>MFCEKAMELIRELHRAPEGQLPAFNEDGLRQVLEEMKALYEQNQSDVNEAKSGGRSDLIPTIKFRHCSLLRNRRCTVAYLYDRLLRIRALRWEYGSVLPNALRFHMAAEEMEWFNNYKRSLATYMRSLGGDEGLDITQDMKPPKSLYIE[2x];>[2x]MDAAEVEFLAEKELVTIIPNFSLDKIYLIGGDLGPFNPGLPVEVPLWLAINLKQRQKCRLLPPEWMDVEKLEKMRDHERKEETFTPMPSPYYMELTKLLLNHASDNIPKADEIRTLVKDMWDTRIAKLRVSADSFVRQQEAHAKLDNLTLMEINTSGTFLTQALNHMYKLRTNLQPLESTQSQDF;>GPHMSEAYFRVESGALGPEENFLSLDDILMSHEKLPVRTETAMPRLGAFFLER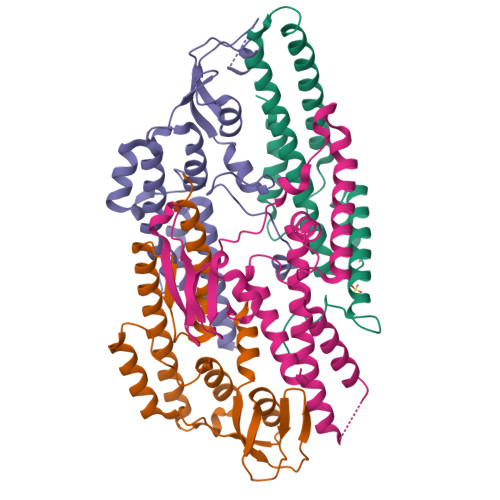SAGAETDNAVPQGSKLELPLWLAKGLFDNKRRILSVELPKIYQEGWRTVFSADPNVVDLHKMGPHFYGFGSQLLHFDSPENADISQSLLQTFIGRFRRIMDSSQNAYNEDTSALVARLDEMERGLFQTGQKGLNDFQCWEKGQASQITASNLVQNYKKRKFTDMED[2x];>MTEEVDFLGQDSDGGSEEVVLTPAELIERLEQAWMNEKFAPELLESKPEIVECVMEQLEHMEENLRRAKREDLKVSIHQMEMERIRYVLSSYLRCRLMKIEKFFPHVLEKEKTRPEGEPSSLSPEELAFAREFMANTESYLKNVALKHMPPNLQKVDLFRAVPKPDLDSYVFLRVRERQENILVEPDTDEQRDYVIDLEKGSQHLIRYKTIAPLVASGAVQLI[2x]>MKDFSKDFLFGVATASYQVEGAYNEDGRTMSIWDTFSRQDGKVYKSHNGDVACDHYHLYKDDVKMMKDLGIEAYRFSIAWPRIFPAKGQYNPKGMDFYKRLTDELLKNDIKPFATIYHWDLPQWADDLGGWLNREIVEWYGEYAEKLFSELGGYIKNWITLNEPWCSSFLSYFIGEHAPGHKDLGEALLVSHNLLLSHGKAVEIFRGLNLDDSKIGITLNLNEVFPASDSDDDKVAAQIADGFQNRWFLDPLFKGKYPQDMVEYFGKYAKVDFINDEDLKLISQKLDFLGVNYYTRAVVQKGNDGLLDAVQIDPGNERTEMGWEIYPESLYNILMRLKREYTYDMPLYITENGAAFNDVVEDDGRVHDEKRVEFLKQHFKEAKRFLNDGGNLKGYFVWSLMDNFEWAHGYSKRFGIVYVDYETEKRILKDSALWYKDLISTRTI[4x]

β-glucosidases (Bgls, β-d-glucopyranoside glucohydrolases, E.C. 3.2.1.21) cleave β-1,4-glycosidic bonds in disaccharides or glucose-substituted polysaccharides, thereby releasing non-reducing terminal glucosyl residues. Bgl proteins have a TIM-barrel fold. The substrate-binding pocket can be divided into the glycone, aglycone, and gatekeeper regions; in addition, the bound sugar substrate is cleaved via a retention mechanism using two glutamate residues. Four loops are present above the Bgl substrate-binding pocket, forming a large cavity for the nascent substrate to access.

Two different space groups of TsaBgl crystals containing triclinic P1 and orthorhombic P212121 were obtained at pH 7.5 and 8.0, respectively. Two TsaBgl-P1 structures were processed up to 1.9 and 2.1 Å, with Rwork/Rfree of 0.1694/0.1952 and 0.1599/0.2019, respectively. The electron density maps of TsaBgl-P1 and TsaBgl-P212121 structures were clearly observed, except for the partially disordered electron density maps between the Gly302 and Gly304 residues in TsaBgl-P1 (chain C and D for Data I and II, respectively). Particularly, the L3 loop exhibited two structurally distinct conformations, one where it was oriented towards the substrate-binding pocket (folded L3 loop) and the other where it was oriented towards the solvent direction, i.e., away from the substrate-binding site (straight L3 loop). Particularly, as both the folded and straight L3 loop conformations were observed within a single crystal in Data I and II, this indicated that the two conformations can appear in the same environment. In the P1 and P212121 crystals, the L3 loop regions of the TsaBgl-Data I (folded L3 loop conformation) and TsaBgl-Data III (straight L3 loop conformation) chain A molecules, which showed the most significant differences in L3 loop conformation, were carefully analyzed. In the top view of the TsaBgl substrate-binding site, the L3 loop in the folded conformation induced a greater narrowing of the substrate-binding pocket than the straight L3 loop and exhibited a relatively negatively charged surface. The substrate accessible width of the substrate-binding pocket entrance with the folded L3 loop conformation was approximately 30 Å, and the proximate distance between the L2 and L3 loops was approximately 5 Å. A Tris molecule was shown to act as an inhibitor of TsaBgl β-glucosidase activity. This molecule was found to bind to all the active sites in the TsaBgl glycone region.> KYEYVELAKASLTSAQPQHFYAVVIDATFPYKTNQERYICSLKIVDPTLYLKQQKGAGDASDYATLVLYAKRFEDLPIIHRAGDIIRVHRATLRLYNGQRQFNANVFYSSSWALFSTDKRSVTQEINNQDAVSDTTPFSFSSKHATIEKNEISILQNLRKWANQYFSSYSVISSDMYTALNKAQAQKGDFDVVAKILQVHELDEYTNELKLKDASGQVFYTLSLKLKFPHVRTGEVVRIRSATYDETSTQKKVLILSHYSNIITFIQSSKLAKELRAKIQDDHSVEVASLKKNVSLNAVVLTEVDKKHAALPSTSLQDLFHHADSDKELQAQDTFRTQFYVTKIEPSDVKEWVKGYDRKTKKSSSLKGASGKGDN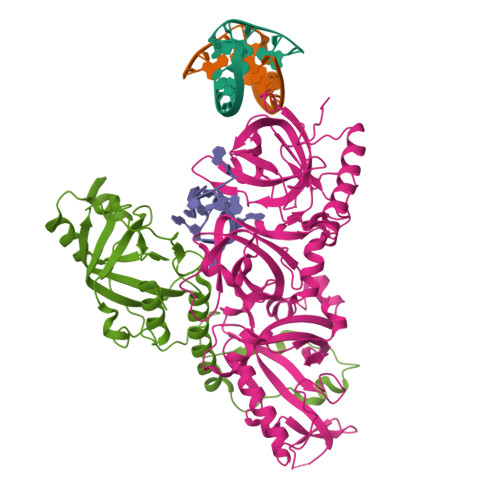IFQVQFLVKDASTQLNNNTYRVLLYTQDGLGANFFNVKADNLHKNADARKKLEDSAELLTKFNSYVDAVVERRNGFYLIKDTKLIY;> QQQSAFKQLYTELFNNEGDFSKVSSNLKKPLKCYVKESYPHFLVTDGYFFVAPYFTKEAVNEFHAKFPNVNIVDLTDKVIVINNWSLELRRVNSAEVFTSYANLEARLIVHSFKPNLQERLNPTRYPVNLFRDDEFKTTIQHFRHTALQAAINKTVKGDNLVDISKVADAAGKKGKVDAGIVKASASKGDEFSDFSFKEGNTATLKIADIFVQEKG>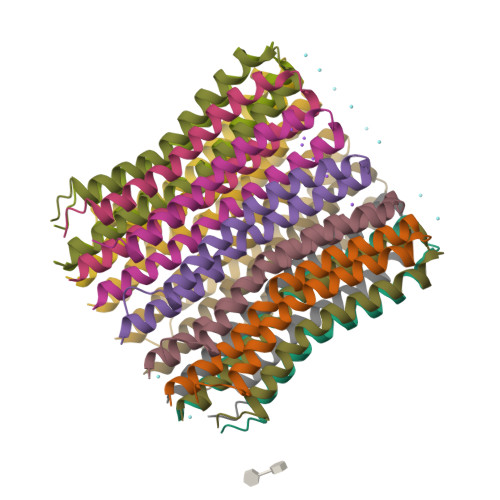PLIAAASVIAAGLAVGLASIGPGVGQGTAAGQAVEGIARQPEAEDKIRGTLLLSLAFMEALTIYGLVVALALLFANPFV[14x]>[3x]MLSVNEIAAEIVEDMLDYEEELRIESKKLENGAIVVDCGVNVPGSYDAGIMYTQVCMGGLADVDIVVDTINDVPFAFVTEYTDHPAIACLGSQKAGWQIKVDKYFAMGSGPARALALKPKKTYERIEYEDDADVAVIALEANQLPDEKVMEFIAKECDVDPENVYALVAPTASIVGSVQISGRIVQTAIFKMNEIGYDPKLIVS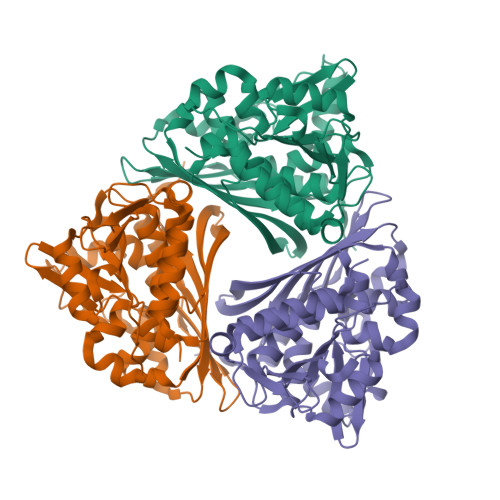GAGRCPISPILENDLKAMGSTNDSMMYYGSVFLTVKKYDEILKNVPSCTSRDYGKPFYEIFKAANYDFYKIDPNLFAPAQIAVNDLETGKTYVHGKLNAEVLFQSYQIVLEE> GIRLKDELINIKQILEAADIMFIYEEEKWPENISLL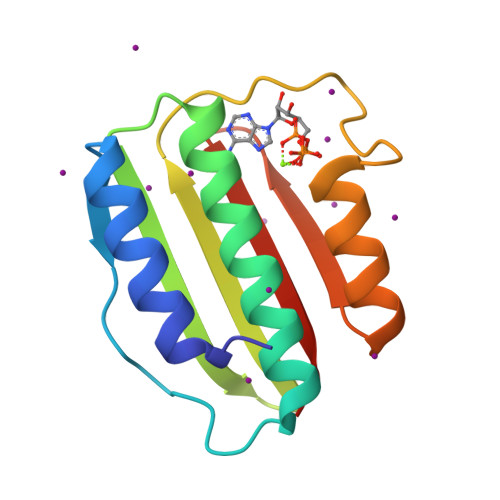NENILSMCLKEAVTNVVKHSQAKTCRVDIQQLWKEVVITVSDDGTFKGEENSFSKGHGLLGMRERLEFANGSLHIDTENGTKLTMAIPNNSK> KPHPWFFGKIPRAKAEEMLSKQRHDGAFLIRESESAPGDFSLSVKFGNDVQHFKVLRDGAGKYFLWVVKFNSLNELVDYHRSTSVSRNQQIFLRDIE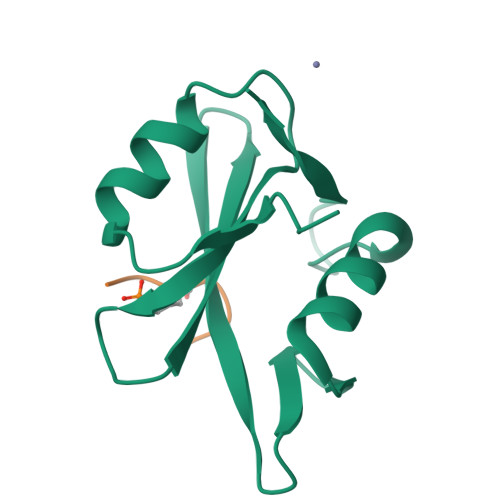Q> GKSASMAVEEIASRKDISLRDMQISAILKMLFLNKDLNNNDNITTITDDIFNQQEIIWKVLILDIKSTATISSVLRVNDLLKAGITVHSLIKQDRSPLPDVPAIYFVSPTKENIDIIVNDLKSDKYSEFYINFTSSLPRNLLEDLAQQVSITGKSDKIKQVYDQYLDFIVTEPELFSLEISNAYLTLNDPKTTEEEITGLCANIADGLFNTVLTINSIPIIRAAKGGPAEIIAEKLGTKLRDFVINTNSSSTSTLQGNDSLERGVLIILDRNIDFASMFSHSWIYQCMVFDIFKLSRNTVTIPLESKENGTDNTTAKPLATKKYDIEPNDFFWMENSHLPFPEAAENVEAALNTYKEEAAEITRKTGVTNISDLDPNSNNDTVQIQEVVKKLPELTAKKNTIDTHMNIFAALLSQLESKSLDTFFEVEQDPGSTKTRSRFLDILKDGKTNNLEDKLRSFIVLYLTSTTGLPKDFVQNVENYFKENDYDINALKYVYKLREFMQLSNMSLQNKSLEDGSDSAFKPSNLTLSGIYGLTEGKLQGGVGSLISGIKKLLPEKKTIPITNVVDAIMDPLNSSQKNLETTDSYLYIDPKITRGSHTRKPKRQSYNKSLVFVVGGGNYLEYQNLQEWAHSQLHNPKKVMYGSTAITTPAEFLNEISRLGASNSSNNDA;> GAMAGMNIKDRTSEFQQSVLSYKKRNKNFREQQRERLQEKESENFA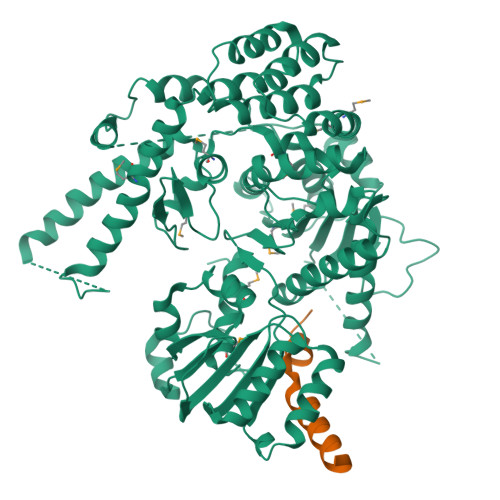NNTT> GSHMASMKKKGSVVIVGRINLSGDTAYAQQTRGEEGCQETSQTGRDKNQVEGEVQIVSTATQTFLATS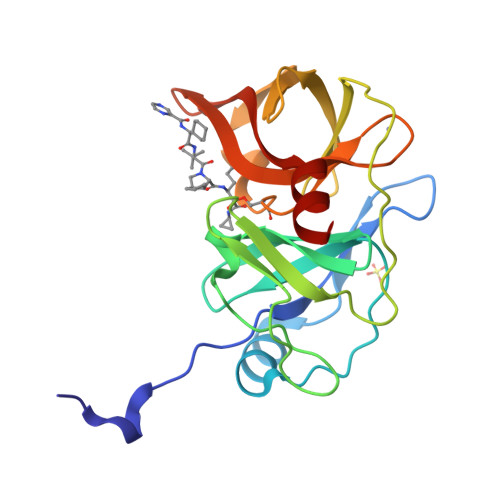INGVLWTVYHGAGTRTIASPKGPVTQMYTNVDKDLVGWQAPQGSRSLTPCTCGSSDLYLVTRHADVIPVRRRGDSRGSLLSPRPISYLKGSSGGPLLCPAGHAVGIFKAAVSTRGVAKAVDFIPVESLETTMRSP>[6x]MHHHHHHGTEKNVFNDAIVEKPNMEPAIPRPEQEKVAVSKLKNLEAKQGRKPNVLVLLVDDLGWGDPGVYGGGAAIGAPTPNIDKLANEGLRLTSMYSQPTCTSSRAALTTGRLPVRSGLVRPILTGDKVTQNP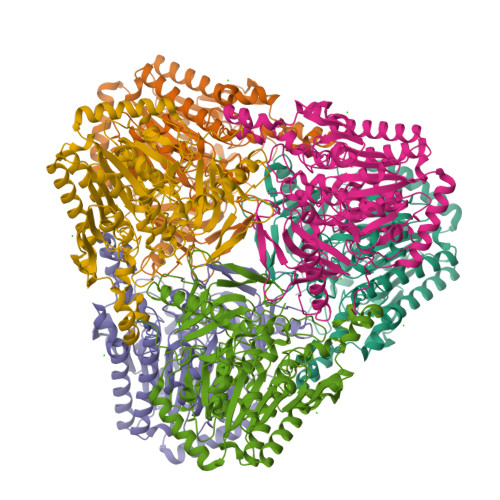WEKEVSQGKLLSKVGYKTALIGKWHVGEAEGMLPHEVGFDYFYGLPSVQSDYTQFLVERQYADMMTNKELYTKASQLRPEGLIKGRKGGKREVAYPINSIEDISMIDQVLRDESVKFINQAVDEGKPFYLIHSFSKIHNDNYPAPKYKGASPAAMPVRDAMVEVDDITGELVALLKEKGQLENTLIIFTSDNGPNEDTWPDSGYSPWRGGKGTTWEGGVRIPGIAYWKGMISAGQVNNGLMDLTDIYMTSLRLGGVIDELPSNMYFDGIDQTAFLLADNGKSRRQVVYMWSREDFTALRWLDYKIHFKVFNTAVPRRNIDASFLLDIGTAPWVFNLNMDPKEMASTGHQYFEWGMPQATKFMKAHIATMKKYPNTDIGLGL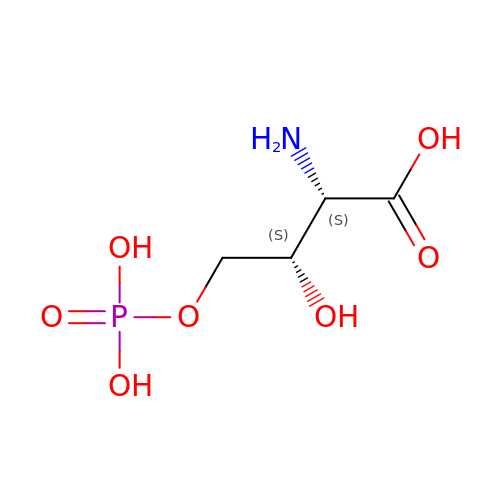4-HYDROXY-L-THREONINE-5-MONOPHOSPHATE | C4 H10 N O7 P | FKHAKIJOKDGEII-GBXIJSLDSA-N> FPTIPLSRLFDNAMLRAHRLHQLAFDTYQEFEEAYIPKEQKYSFLQNPQTSLCFSESIPTPSNREETQQKSNLELLRISLLLIQSWLEPVQFLRSVFANSLVYGASDSNVYDLLKDLEERIQTLMGRLEDGSPRTGQIFKQTYSKFDTNSHNDDALLKNYGLLYCFRKDMDKVETFLRIVQCRSVEGSCGF;> FSGSEATAAILSRAPWSLQSVNPGLKTNSSKEPKFTKCRSPERET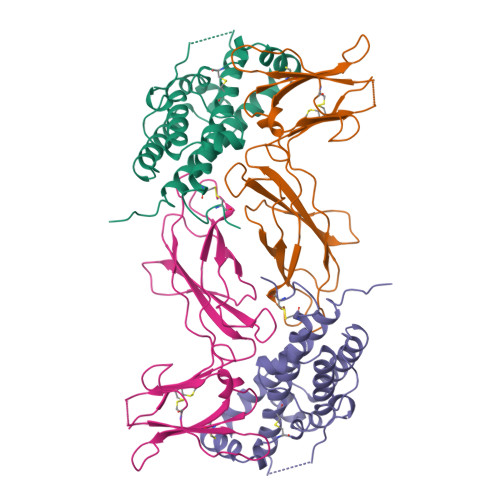FSCHWTDEVHHGTKNLGPIQLFYTRRNTQEWTQEWKECPDYVSAGENSCYFNSSFTSIWIPYCIKLTSNGGTVDEKCFSVDEIVQPDPPIALNWTLLNVSLTGIHADIQVRWEAPRNADIQKGWMVLEYELQYKEVNETKWKMMDPILTTSVPVYSLKVDKEYEVRVRSKQRNSGNYGEFSEVLYVTLPQMS>XGEIA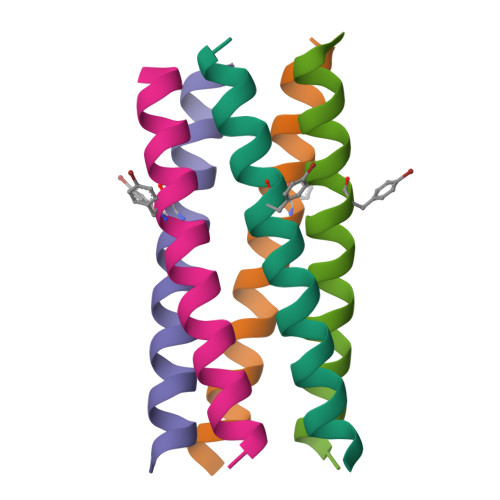QTLKEIAKTLKEIAYTLKEIAQTLKGX[5x]> GAMGSTIARTIVLQESIGKGRFGEVWRGKWRGEEVAVKIFSSREERSWFREAEIYQTVMLRHENILGFIAADNKDNGTWTQLWLVSDYHEHGSLFDYLNRYTVTVEGMIK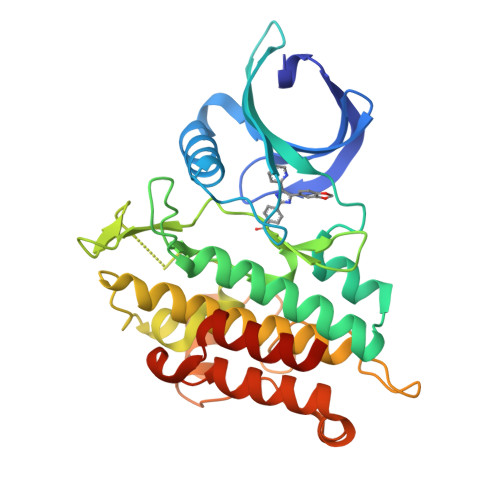LALSTASGLAHLHMEIVGTQGKPAIAHRDLKSKNILVKKNGTCCIADLGLAVRHDSATDTIDIAPNHRVGTKRYMAPEVLDDSINMKHFESFKRADIYAMGLVFWEIARRCSIGGIHEDYQLPYYDLVPSDPSVEEMRKVVCEQKLRPNIPNRWQSCEALRVMAKIMRECWYANGAARLTALRIKKTLSQLSQQEGIKM>MPFQQGLLATPVPAHARHLFFTLQSPEALPAALDALLPQVDGKQLLLGVGAPLAKALGREIPGLRPFPLLDAAVENPSTQHALWLWLRGDERGDLLLRTQALEQALAPALSLADSVDGFLHRGGHDLTGYEDGTENPTDEEAVQAAIAADGSSFAAFQLWKHDLQYFKSLPQADQDNIIGRRLSDNEELDDAPASAHVKRTAQESFEPEAFMVRRSVSWADQRGAGLAFVALGKSFEAFEVQLRRMSGLEDGIIDGLYRFSRPLTGGYYWCPP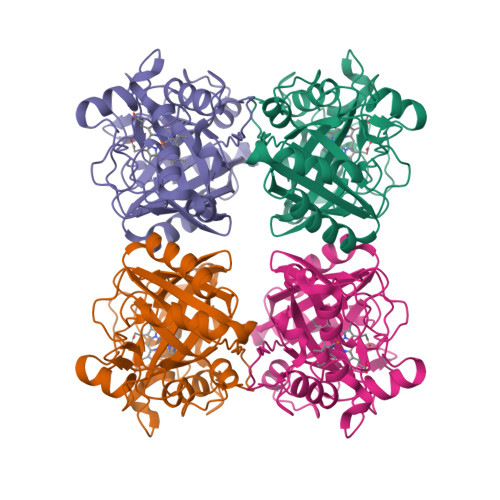MSETGVDLSPLLRA[4x]> SNAVAARTLPDRFIARAPVPADAPAIARLIAACQEADGDEPDASAEEVLRDWEGLDLGQEAVLVVAPDGEAAAYADVLNRRYVQLSVYGYVHPRFRGMGLGTWLVQWGEEWIQDRMHLAPAEAQVTVQHYIRASSTSALRLMEQHGYRPVRDIWVMAITLDQPPPAPEWPEGITARTFVPGLDERATYEAVEEAFGDIWGRPPSTFERWLSMTQSERKDPELWLLAVETDSGHIVGTCLGQETAGKGWIGSVGVRRPWRGRGIALALLQEVFGVYYRRGVREVELSVDAESRTGAPRLYRRAGMHVKHRYVLHRKEIRPGIDLS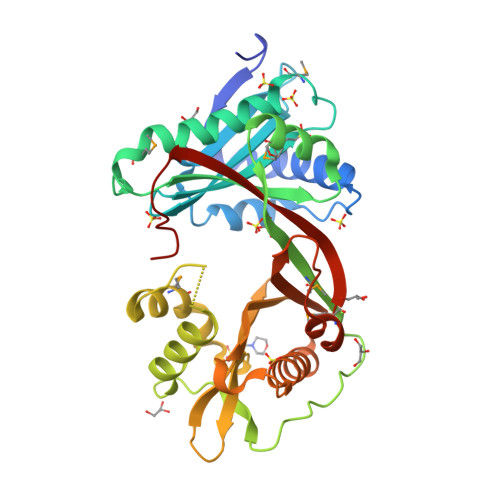TTAAHS DIAMIDOPHOSPHATE | H5 N2 O2 P | 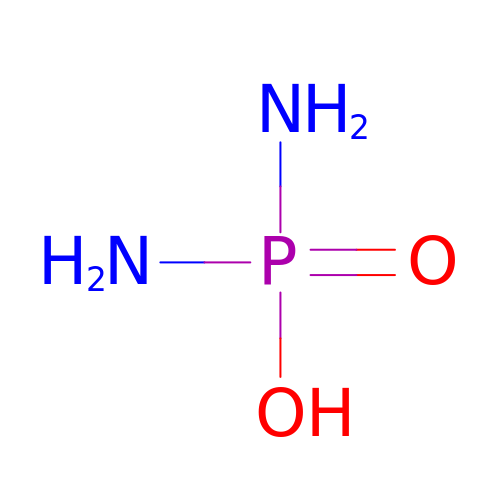ANCLJVISBRWUTR-UHFFFAOYSA-N(5R,7R,8S,9S,10R)-7-(hydroxymethyl)-3-phenyl-1,6-dioxa-2-azaspiro[4.5]dec-2-ene-8,9,10-triol | C14 H17 N O6 | 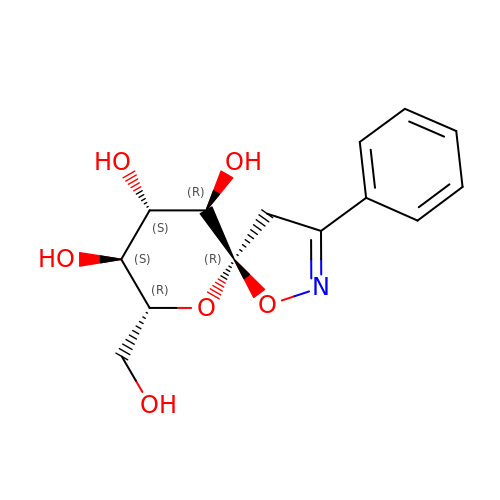YLTDNVVQKRHCJP-RKQHYHRCSA-N> GSGSAMIEARQVSELSTRIISSVQMLSNAQNEQERKEAGRVLFEQLESLLTHIKELGGESFDSKLLDALESNVQNVINNLAELGVTVERKLWLAKEIDT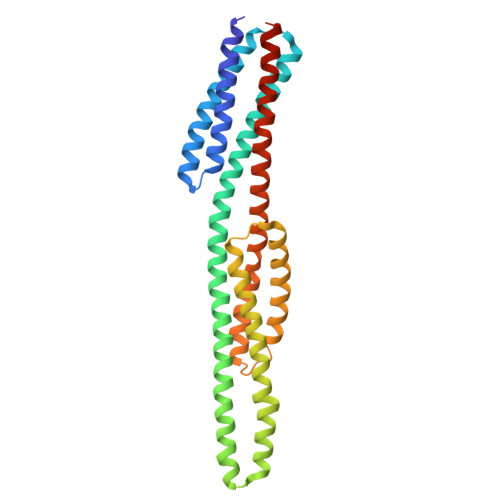RVEEMRLLSEELEQLTRTQVQNTSTIAVANVTHIYDLLEANKKDQVYQALDALVEVDLDLTERLHELHLLAFKMLNQIEEARTLTNVDRIQQIQTAFENNLKIMKRRVLAVEDPTRSKQMSQLLTELGKRQVVFTILLQQYENNEQSQQLMQKTLELFSELNSTVNKLVDDSNKTTTK3-METHYL-4-PHENYL-1H-PYRAZOLE | C10 H10 N2 | 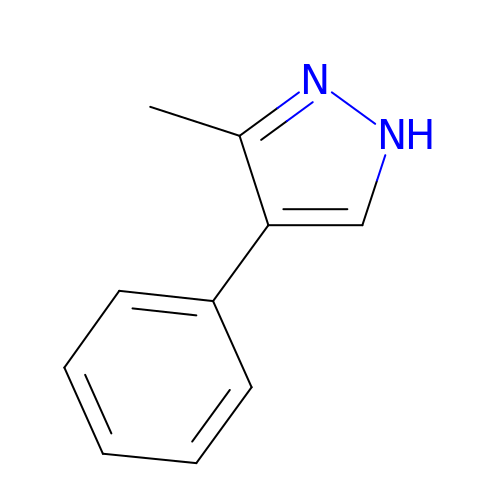XTXZCNATVCIKTR-UHFFFAOYSA-N>[2x]PDPNRFDRDRLFNAVSRGVPEDLAGLPEYLSKTSKYLTDSEYTEGSTGKTCLMKAVLNLKDGVNACILPLLQIDRDSGNPQPLVNAQCTDDYYRGHSALHIAIEKRSLQCVKLLVENGANVHARACGRFFQKGQGTC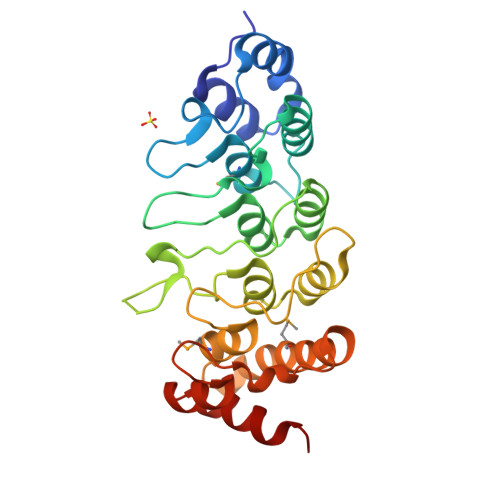FYFGELPLSLAACTKQWDVVSYLLENPHQPASLQATDSQGNTVLHALVMISDNSAENIALVTSMYDGLLQAGARLCPTVQLEDIRNLQDLTPLKLAAKEGKIEIFRHILQREFS> EAGGVFKLIANDGKADRMIMANDLLNDRIKSIMCLRAKQGFSDPTPTLVDIERTHILLINSHYKPFAAMGYEYQKTRPNTGNPTYNSTIQFSIPQFGDFFSDMVVHVQLAATSASAGTVPALPAFIGADDQVLTSTSVVSATENTTSGVYTLYTQSYVNQQGTTQTVAAAATNFVRYCEYPGLRLFKRVKFEVNGNPLDEYTALAAIMYNKFHVPDFKLTGWKRLIGQEVPVEAASNLVNIASTTPWGSPIVALSDVNGTAVTGSPVNAA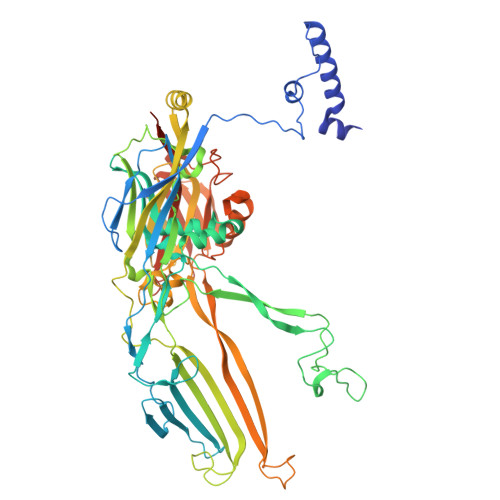ITARKLTQVVFGAQTPKATQEQLNMFVPLLFWFRDPRLAIASVSIPYGQRFITVDIEQQSNILFTAPGNLFLQTTVETLLTTGAGKGTATGVLLTQYNRYTTYTPTLASGSSIDGTQAVQNIELYINNIFVTPEIHDIYIKRIGFTLIRVYREQVQREVNAADQVLQSQLKWPVEFIYLGLRPANNIAAGNTYQWRDWHHLTSVTNEPVYDVSQSYARVSIDDTVAPVGSTTFKQSASQVMQNQYIVPVETETLDTVRVKAHGIELYAQYRAQFYRDYIPWNYGSFNLVTPQDKGALFLNFCLYPGTYQPSGHVNISRAREFYIEYTSSFCDSSNPCDLISIAKCINFLLISDGSAVLRYSTKEFYLQCLILRCI>MHHHHHHTQHGIRLPLRSGLGGAPLGLRLPRETDEEPEEPGTTGSFVEMVDNLRGKSGQGYYVEMTVGSPPQTLNILVDTGSSNFAVGAAPHPFLHRYYQRQLSSTYRDLRKGVYVPYTQGKWEGELGTDLVSIPHGPNVTVRANIAAITESDKFFINGSNWEGILGLAYAEIARPDDSLEPFFDSLVKQTHVPNLFSLQLCGAGFPLNQSEVLASVGGSM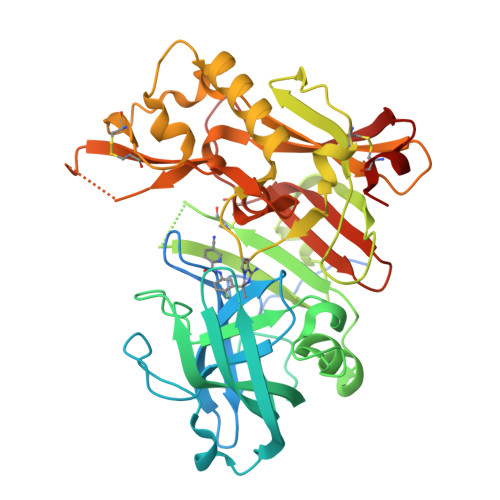IIGGIDHSLYTGSLWYTPIRREWYYEVIIVRVEINGQDLKMDCKEYNYDKSIVDSGTTNLRLPKKVFEAAVKSIKAASSTEKFPDGFWLGEQLVCWQAGTTPWNIFPVISLYLMGEVTNQSFRITILPQQYLRPVEDVATSQDDCYKFAISQSSTGTVMGAVIMEGFYVVFDRARKRIGFAVSACHVHDEFRTAAVEGPFVTLDMEDCGYN[3x]>[3x]PIATPYPVKEWLQPKRYKAHLMGTTYVYDFPELFRQASSSQWKNFSADVKLTDDFFISNELIEDENGELTEVEREPGANAIGMVAFKITVKTPEYPRGRQFVVVANDITFKIGSFGPQEDEFFNKVTEYARKRGIPRIYLAANSGARIGMAEEIVPLFQVAWNDAANPDKGFQYLYLTSEGM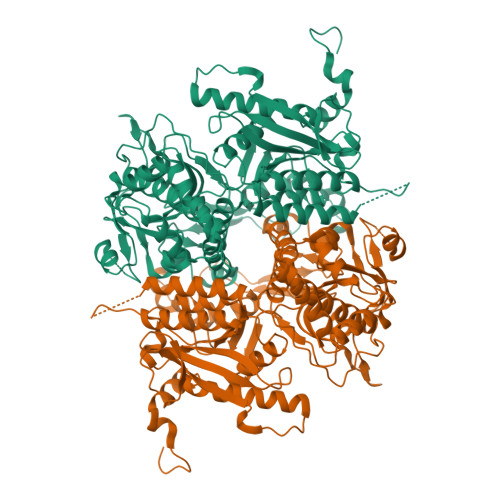ETLKKFDKENSVLTERTVINGEERFVIKTIIGSEDGLGVECIRGSGLIAGATSRAYHDIFTITLVTCRSVGIGAYLVRLGQRAIQVEGQPIILTGAPAINKMLGREVYTSNLQLGGTQIMYNNGVSHLTAVDDLAGVEKIVEWMSYVPAKRNMPVPILETKDTWDRPVDFTPTNDETYDVRWMIEGRETESGFEYGLFDKGSFFETLSGWAKGVVVGRARLGGIPLGVIGVETRTVENLIPADPANPNSAETLIQEPGQVWHPNSAFKTAQAINDFNNGEQLPMMILANWRGFSGGQRDMFNEILKYGSFIVDALVDYKQPIIIYIPPTGELRGGSWVVVDPTINADQMEMYADVNARAGVLEPQGMVGIKFRREKLLDTMNRLDDKYRELRSQLSNKSLAPEVHQQISKQLADRERELLPIYGQISLQFADLHDRSSRMVAKGVISKELEWTEARRFFFWRLRRRLNEEYLIKRLSHQVGEASRLEKIARIRSWYPASVDHEDDRQVATWIEENYKTLDDKLKGLKLESFAQDLAKKIRSDHDNAIDGLSEVIK> MNHKVHMGRSQNSEFETASDEPIAVIGLSCRLPKASGPQELWQLLDDGASAVTRVPADRETPPSTEEESADGEAAGARWGGFLDRVDTFDAGFFGISPREAAAMDPQQRLVLELSWEALEGAGLVPATLRDTGLGVFVGAARDDYATLYRRREGRAVDHHAMTGLHRSLIANRISYALGAHGPSMVVDTGQSSSLVAVHLACESLRRGESDIALAGGVNLNIAAESARETAAFGGLSPDGQCFTFDARANGFVRGEGGGLVVLKTLRRALADGDLVHGVILASAVNNDGPSDTLTTPSRRAQESLLTRVYRRAGVTPTEVGYVELHGTGTKVGDPIEAAALGAVLGTGRDTPLPVGSIKTNIGHLEGAAGIAGLIKALLQLRRRRLVPSLNFSTPNPDIPLDALNLRVQQESAPWATPSGGGRTLVAGVSSFGMGGTNCHVVVSAAPVPEDGETTSEAGATGPDSGPALLPWVVSARSPQALRDQAGRLAAWADSPAGREASPVDIGWSLATSRTHFEYRAVVSGSDRDELVASLRALASGSPVTAAGAVDGGGRLGLVFSGQGSQRAGMGRELYVAFPVFAEAFDEVCGVLDEVMGALPPSEGWAGSLREVMFEVSSDLLDETGFTQPALFAFEVALYRLLESWGVAGEVVAGHSVGEIAAVHVAGVLSLADACALVAARGRLMQGLPSGGAMVAVEASEEEVTALLAGREGEVGIGAVNGPRSVVVSGGVAVVEEVAAHFAGLGRRARRLKVSHAFHSPLMDPMLEDFGRVVAGLSFAVPELTVVSGLTGAVVSADELCSVGYWVRHAREAVRFADAVGAMAGVGVGRFVEVGPGGVLSALVRECLAEGGAGSVVAAVRGNRAEPVALLSAVGELFADGYPVD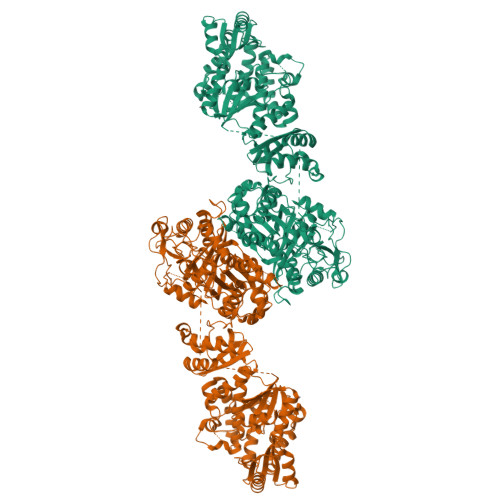WTAYFAGWPAARVELPTYAFQRSRHWLENVPELAVS> VHFAPTITFLESPTSDHHWCIPFTVKGNPKPAL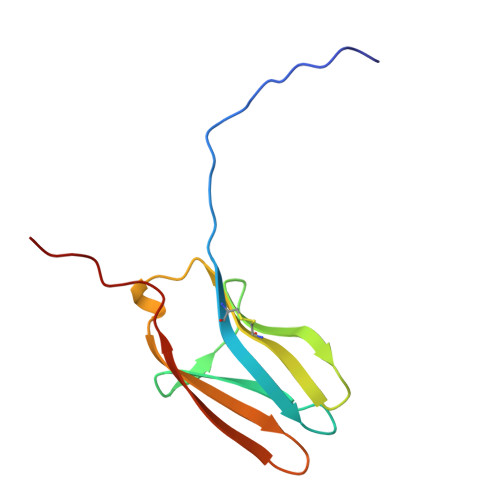QWFYNGAILNESKYICTKIHVTNHTEYHGCLQLDNPTHMNNGDYTLIAKNEYGKDEKQISAHFMGWPGID3,3'-[3,5-DIFLUORO-4-METHYL-2,6-PYRIDYLENEBIS(OXY)]-BIS(BENZENECARBOXIMIDAMIDE) 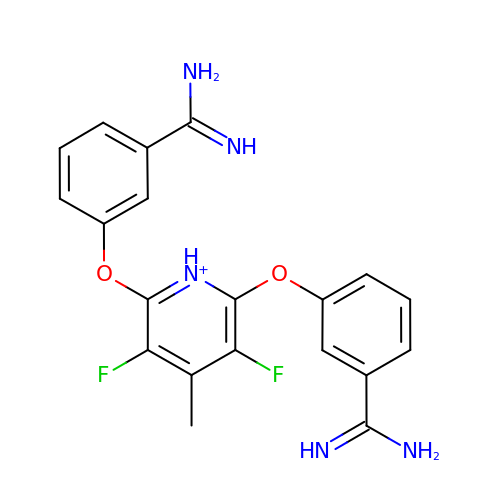| C20 H18 F2 N5 O2 | ZXIHYCYAQUQHSG-UHFFFAOYSA-O6-AMINOPYRIMIDIN-2(1H)-ONE | C4 H5 N3 O | 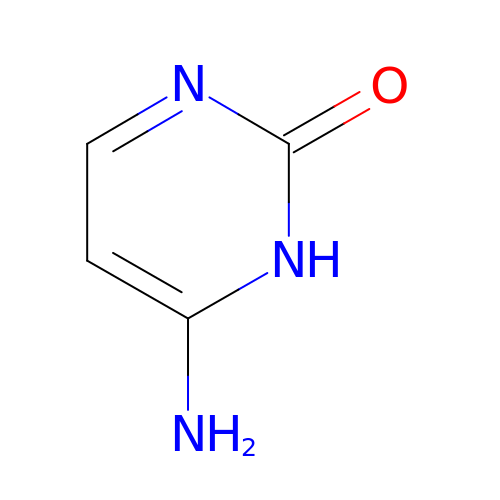OPTASPLRGRRNAP-UHFFFAOYSA-N The NAD(P)+-dependent succinate semialdehyde dehydrogenase (SSADH) Sad is a member of the ALDH superfamily and oxidizes succinate semialdehyde (SSA) to succinate. In microorganisms, SSADHs operate in the degradation of various nitrogen-containing compounds such as putrescine or arginine, where they prevent the accumulation of the toxic SSA intermediate. Our results show that Sad is a surprisingly flexible enzyme that is not only able to detoxify succinate semialdehyde and glutarate semialdehyde but can also functionally substitute erythrose 4-phosphate dehydrogenase in pyridoxal 5′-phosphate (PLP) biosynthesis and glyceraldehyde 3-phosphate dehydrogenase (as well as phosphoglycerate kinase) in glycolysis under physiological conditions. We show that Sad, which primarily functions in the detoxification of succinate semialdehyde in various degradation pathways, does not only accept closely related substrates, but also converts phosphorylated sugars as a side reactivity.

EG2.2s had acquired a non-synonymous substitution in sad, resulting in an amino acid change of Q262R; while EG2.3a, EG2.4a, and EG2.5a were predicted by the breseq pipeline28 to carry amplified genomic regions that encoded sad (~80×). To understand the molecular basis of the improved enzyme activity in the Q262R variant, we solved the crystal structures of both Sad WT and Q262R variants with bound NAD+, as well as in complex with both NAD+ and SSA. While we were not able to obtain structures with sufficient electron densities for the alternative sugar-phosphate substrates, we manually fitted E4P and GAP based on the NAD+/SSA-bound structures. Potential interactions for the coordination of SSA are shown as black dashed lines and important distances are given in Å. f, g The active site of the Q262R variant of Sad with bound NAD+ and modeled E4P & GAP (based on the position of SSA in the Q262R variant, taking into account available space and potential coordinating residues). R262 is likely responsible for an improved coordination of the phosphate group of E4P and GAP. Moreover, in the Q262R variant, E4P dehydrogenase activity was increased 17-fold compared to the WT, reaching 800 nmol min−1 mg−1. Further kinetic investigations revealed that the Q262R substitution had significantly improved the Km of Sad for sugar phosphates. Km, its affinities toward E4P and GAP were increased by 75- and 16-fold, respectively. This improved the catalytic efficiency of the reaction with E4P and GAP by two orders of magnitude, reaching kcat/Km-values that fall in the range of enzymes on their native substrates (103−108 s−1 M−1). In contrast, in the EG2.2s strain that harbored the Sad Q262R variant, the Sad expression level was unchanged, supporting the finding that the single amino acid substitution was sufficient to increase E4P dehydrogenase flux.

>[4x]MTITPATHAISINPATGEQLSVLPWAGADDIENALQLAAAGFRDWRETNIDYRAEKLRDIGKALRARSEEMAQMITREMGKPINQARAEVAKSANLCDWYAEHGPAMLKAEPTLVENQQAVIEYRPLGTILAIMPWNFPLWQVMRGAVPIILAGNGYLLKHAPNVMGCAQLIAQVFKDAGIPQGVYGWLNADNDGVSQMIKDSRIAAVTVTGSVRAGAAIGAQAGAALKKCVLELGGSDPFIVLNDADLELAVKAAVAGRYRNTGQVCAAAKRFIIEEGIASAFTERFVAAAAALKMGDPRDEENALGPMARFDLRDELHHQVEKTLAQGARLLLGGEKMAGAGNYYPPTVLANVTPEMTAFREEMFGPVAAITIAKDAEHALELANDSEFGLSATIFTTDETQARQMAARLECGGVFINGYCASDARVAFGGVKKSGFGRELSHFGLHEFCNIQTVWKDRI> PFAQIYILEGRTPEQKKAVIEKVTQALHEATDAKKETIRVWIHEMPKENWGIAGVSAKDLGRL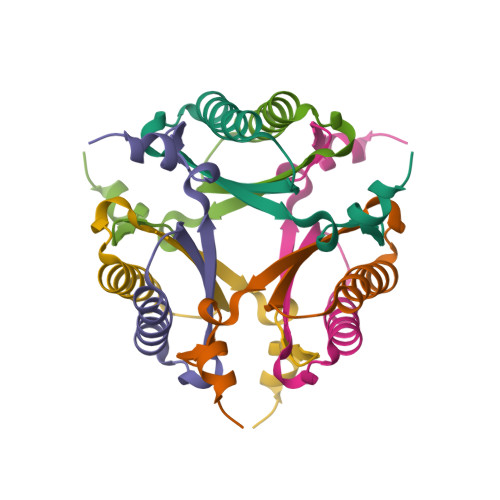EHHHHHH> DRLDCVKASDQCLKEQSCSTKYRTLRQCVAGKETNFSLASGLEAKDECRSAMEALKQKSLYNCRCKRGMKKEKNCLRIYWSMYQSLQGNDLL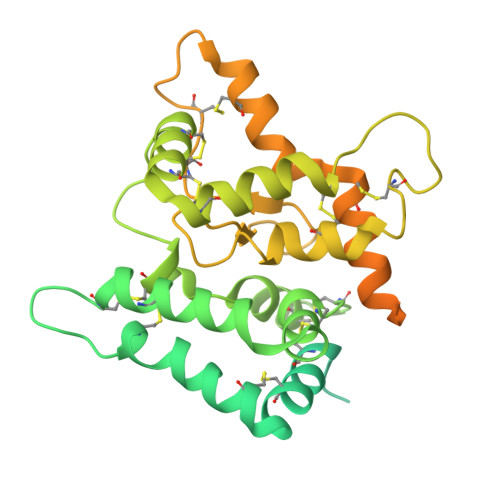EDSPYEPVNSRLSDIFRVVPFISDVFQQVEHIPKGNNCLDAAKACNLDDICKKYRSAYITPCTTSVSNDVCNRRKCHKALRQFFDKVPAKHSYGMLFCSCRDIACTERRRQTIVPVCSYEEREKPNCLNLQDSCKTNYICRSRLADFFTNCQPESRSVSSCLKENYADCLLAYSGLIGTVMTPNYIDSSSLSVAPWCDCSNSGNDLEECLKFLNFFKDNTCLKNAIQAFGNGSDVTVWQPAFPVQTTTATTTTALRVKNKPLGPAGSENEIPTHVLPPCANLQAQKLKSNVSGNTHLCISNGNYEKEGLGGTHHHHHHHH> 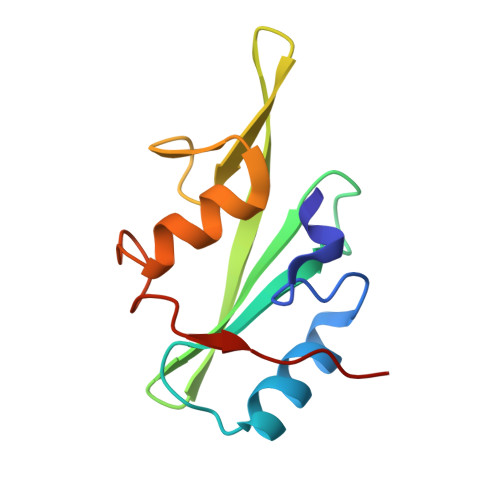IHRTQHWFHGRISREESHRIIKQQGLVDGLFLLRDSQSNPKAFVLTLCHHQKIKNFQILPCEDDGQTFFSLDDGNTKFSDLIQLVDFYQLNKGVLPCKLKHHCIRVAL>[2x]SSMEIRVRVEKDPELGFSISGGVGGRGNP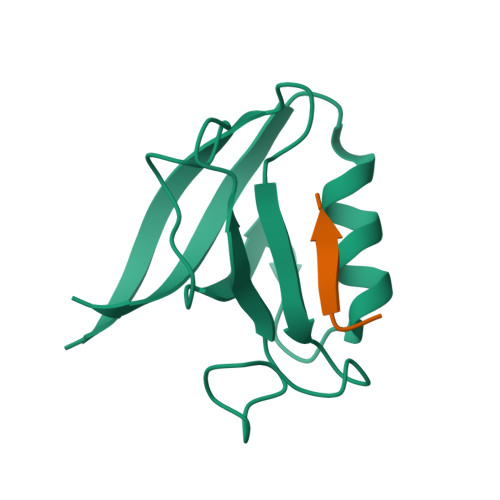FRPDDDGIFVTRVQPEGPASKLLQPGDKIIQANGYSFINIEHGQAVSLLKTFQNTVELIIVREV;>[2x]TGYETWV>MFIKPGRCPKPAVQEDFDAARYLGVWYDIQRLPNKFQKGECATATYSLSPGVGFSVFNRERLANGTIKSVIGSAIAEDPCEPAKLQFFHENAAPVPYWVLSTDYDNYALVYSCINLGASHAAYASIVSRQPTLPEETIKKLQGTMSSFGVGVDTLLTTNQD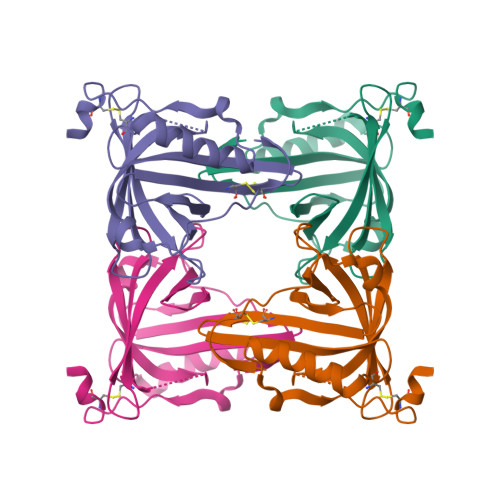AAYCSAMNQKLAAALEHHHHHH[2x]> MDVSILGTGLMGTALAQALIRSGTKVTVWNRTADRALPL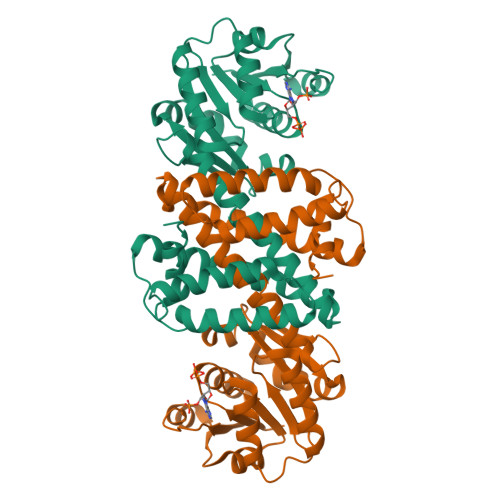AAAGATVAESPQSAIAASPLIVISLLNYEIAKDVVTEADSIAGKIIVNTATGTPEEANQFAEWIAGRGARYLDGAIAAYPEDIGTESSGINYSGDEDVWEDVQSLLTPIAAQSRYVGARPGAANVIDAAMAGAFFNVALGAFHEAAAYVRSEDVAIAEMRHSLHLWTDKLLELLHEALKAFESGEYETDQATLNVYAAAVEAWQQSMQRAGQRAALMTANLDNLQRACAAGHGDKGIFAQIETLSANPQSAI>MAHHHHHHVGTFENITAAPADPILGLADLFRADERPGKINLGIGVYFDETGKIPVLTSVKKAEQYLLENETTKYYLGIDGIPEFGRCTQELLFGKGSALINDKRARTAQTPGGTGALRVAADFLAKNTSVKRVWVSNPSWPNHKSVFNSAGLEVREYAYYDAENHTLDFDALINSLNEAQAGDVVLFHGCCHNPTGIDPTLEQWQTLAQLSVEKGWLPLFDFAYQGFARGLEEDAEGLRAFAAMHKELIVASSYSKNFGLYNERVGACTLVAADSETVDRAFSQMKAAIRANYSNPPAHGASVVATILSNDALRAIWEQELTDMRQRIQRMRQLFVNTLQEKGANRDFSFIIKQNGMFSFSGLTKEQVLRLREEFGVYAVASGRVNVAGMTPDNMAPLCEAIVAVL[2x]

E. coli aspartate aminotransferase (AAT) is a pyridoxal phosphate (PLP)-dependent enzyme that catalyses the reversible transamination of l-aspartate with α-ketoglutarate, yielding oxaloacetate and l-glutamate. During its catalytic cycle, AAT undergoes hinge movement to switch between an open conformation, in the ligand-free form, and a closed conformation upon association with substrates or inhibitors. Using our approach, we enrich the less populated but catalytically active closed conformation in order to increase catalytic efficiency (kcat/KM) with the non-native substrate l-phenylalanine, leading to altered substrate selectivity. Steady-state kinetics reveal kcat/KM increases of up to 100-fold towards this aromatic amino acid, resulting in a selectivity switch of up to 1900-fold, and structural analyses by room-temperature X-ray crystallography and multitemperature nuclear magnetic resonance (NMR) spectroscopy confirm that the conformational landscape is remodeled to favor the target state.

To obtain structures in the absence of maleate, we applied a rigorous crystal soaking method to serially dilute and extract the inhibitor from the crystallized enzymes. Superposition of bound and unbound structures for each variant confirmed that closed library mutants VFIT and VFIY remained in the closed conformation in the inhibitor-free form, similar to HEX, while OpenLow variant VFCS and OpenHigh variant AIFS adopted the open conformation, similar to WT. Overlay of AAT structures (Chain A) in the presence and absence of maleate show transition from open to closed states upon inhibitor binding for WT, VFCS, and AIFS, but not for HEX, VFIT, and VFIY, which already adopt the closed conformation in the absence of bound inhibitor. We next analyzed two mutants from the Closed library (VFIT and VFIY). 19F NMR spectra at 278 K for both mutants showed a narrow peak centered at approximately ‒60.2 ppm that is similar to that of WT. Spectra of these variants also showed another broad peak centered at approximately ‒61.2 ppm that is similar to the HEX peak characteristic of the closed conformation. The relative intensity of the two peaks showed similar temperature dependence, with an increase in the relative intensity of the WT-like peak as temperature was increased to 308 K. Peak deconvolution and integration were used to evaluate the population of the two states, and confirmed that at low temperatures both VFIT and VFIY favor the state resembling that adopted by the closed HEX mutant (T < 288 K or 283 K, respectively). However, unlike HEX, at higher temperatures the alternate conformation with the WT-like peak becomes the favored state. Interestingly, ΔE values for these mutants were smaller in magnitude than that calculated for HEX, supporting the predictive nature of the calculated energy differences between open and closed states for these sequences.>[2x]MRVLGIETSCDETGIAIYDDEKGLLANQLYS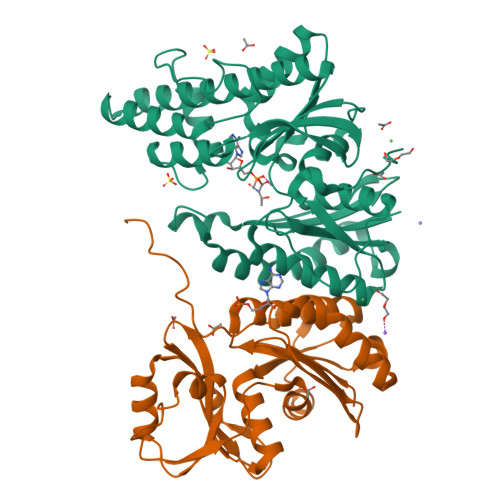QVKLHADYGGVVPELASRDHVRKTVPLIQAALKESGLTAKDIDAVAYTAGPGLVGALLVGATVGRSLAFAWDVPAIPVHHMEGHLLAPMLEDNPPEFPFVALLVSGGHTQLISVTGIGQYELLGESIDDAAGEAFDKTAKLLGLDYPGGPLLSKMAAQGTAGRFVFPRPMTDRPGLDFSFSGLKTFAANTIRDNGTDDQTRADIARAFEDAVVDTLMIKCKRALDQTGFKRLVMAGGVSANRTLRAKLAEMMKKRRGEVFYARPEFCTDNGAMIAYAGMVRFKAGATADLGVSVRPRWPLAELPAAHHHHHH;>[2x]MRILAIDTATEACSVALWNDGTVNAHFELCPREHTQRILPMVQDILTTSGTSLTDINALAYGRGPGSFTGVRIGIGIAQGLALGAELPMIGVSTLMTMAQGAWRKNGATRVLAAIDARMGEVYWAEYQRDENGIWHGEETEAVLKPEIVHERMQQLSGEWVTVGTGWQAWPDLGKESGLVLRDGEVLLPAAEDMLPIACQMFAEGKTVAVEHAEPVYLRNNVAWKKLPGKEHHHHHH>GGSLINFTDGFESTGVNQQPSGWGNFVGWQSNNPNNNIGQSVYALVDNTRAFTGNNSVHFKGGAAPAQIVRTLPAGLDKVYLKAMVYMSKKLGNEAGDNHEHIFGVRGNVAQADNEVRFGQIKGHVGTNEMPSDDISPPQSQWYSGPEIAADTWHCVVVEMLGGNRPYHQLHAYLDNQLIHSIDSISDWNNGGVNGNTQWLDGKLNYAFFGWHSFSNNNADVWMDDIEISDQPISCDSRELEHHHHHH[2x]

We therefore set out to characterize two previously unstudied proteins from the shipworm symbiont Teredinibacter turnerae that were initially identified by the presence of carbohydrate binding domains appended to uncharacterized domains with probable redox functions. One of these was TERTU_3803, which contained both a CBM10 and a CBM2 domain attached to a range of distinct modules (via flexible linkers) that did not bare any sequence similarity with catalytic domains typically found within carbohydrate-active enzymes. Using a ‘module walking’ approach, we searched for other genes coding for these X-domains. This led to the identification of TERTU_2913, which lacks CBMs but contains predicted X122, X183 and X132 domains. Taken together, these sequence analyses suggested that TERTU_3803 and TERTU_2913 could have a role to play in cellulose metabolism, and furthermore that role is likely to be a redox one given the presence of cytochrome domains within their linear amino acid sequences.

In addition to our work on Ttpf08450-X173, we produced TtX122A and TtX122B, representing the X122 domains from TERTU_3803 and TERTU_2913, respectively. The electron density was readily interpretable allowing two molecules of TtX122A to be modelled in the asymmetric unit without breaks in the chain representing residues 3 to 244 of the protein coded for in our construct. Three molecules of TtX122B were present in the asymmetric unit, with chain B’s electron density most readily traced allowing modelling of residues 2 to 235 without breaks in the chain. Chains A and C had some areas that displayed more disorder, so there were breaks in the model between residues 190 and 192 in chain A and residues 162 and 165 in chain C. In addition to protein and water molecules, two magnesium ions were modelled into the electron density on each protomer in TtX122A based on coordination geometry and bond lengths [Fig. S4(a)]; these ions presumably bound from the crystallization medium. Our subsequent structural analysis therefore focused on single protomers from each structure. The overall structures of TtX122A and TtX122B reveal that these domains adopt a β-jelly-roll fold [Figs. 4(a) and 4(b)]. Since there was limited functional similarity between the proteins identified in our structural comparisons, we performed a sequence alignment of 648 X122 family members and mapped the sequence conservation of each amino acid onto the surface of TtX122A using the ConSurf server. This revealed two significantly conserved patches on the protein surface [Fig. 4(c)], one of which was located around the calcium binding site implicated in stabilizing the fold, whilst the other forms a conserved surface on the inner face of the β-jelly-roll fold centred around Arg118 [Fig. 4(d)].>[12x]XGEIAQAFKEIAKAFKEIAWAFKEIAQAFKGX

CCs are quaternary structures comprising two or more α-helices supercoiled around each other with cyclic (Cn) or dihedral (Dn) symmetry. Here, we describe variants with all combinations of the aliphatic residues, Ile, Leu and Val, at a and d to give four classes of peptide: the ββ class, with a and d = Ile or Val; Lβ, a = Leu and d = Ile or Val; βL, a = Ile or Val and d = Leu; and LL, a = d = Leu. Peptides are named systematically appending the one-letter code for the amino acids at the a and d sites to “CC-Type2-“; e.g., CC-Hept becomes CC-Type2-LI. In summary, solution-phase data and X-ray crystal structures demonstrate conclusively that different classes of Type-2 coiled-coil (CC) peptides—i.e., based on abcdefg repeats with predominantly hydrophobic residues at a, d, e and g—adopt a range of distinct states.

Extending the sp2 hybridisation with Leu→Phe mutations gave CC-Type2-FI, which, by X-ray crystallography, formed a 6-helix collapsed structure similar to CC-Type2-LL. Thus, the additional bulk and hydrophobicity of Phe overrides d = Ile and drives collapse of a consolidated core. However, the large Phe residues are accommodated through a half-heptad translation along the superhelical axis between the two helical sheets, resulting in 21 screw symmetry. Despite the complexity of these Phe-containing structures, they are CCs founded on KIH packing. Moreover, the KIH analysis revealed that helices with the same sequence participate in different quaternary arrangements. Similarly, the sequences with bulky Phe at a or d fit poorly to most structures other than their own.> MMITLDHVTKQY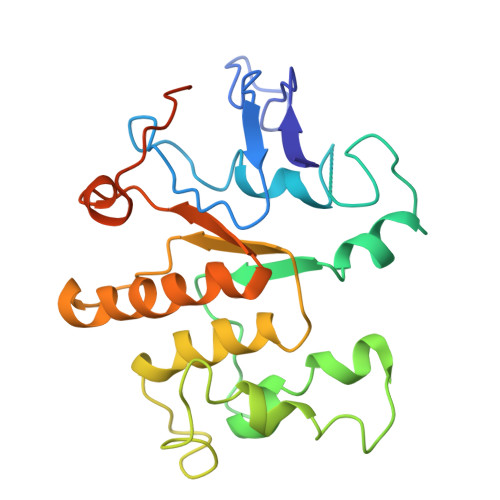KSSARPALDDINVKIDKGEFVFLIGPSGSGKSTFMRLLLAAETPTSGDVRVSKFHVNKLRGRHVPKLRQVIGCVFQDFRLLQQKTVYDNVAFALEVIGKRTDAINRVVPEVLETVGLSGKANRLPDELSGGEQQRVAIARAFVNRPLVLLADEPTGNLDPETSRDIMDLLERINRTGTTVLMATHDHHIVDSMRQRVVELSLGRLVRDEQRGVYGMDR> MSVPITRSLQFLRAVHSWLKIARLRSGSYSKLHVTIFRSTPMIRDIIRMGDKRLLRVAPQVTNLGSAELHALVSDMFETMGAAHGVGLAAPQIAVDLQLMVFGFEASERYPEAPAVPLTALANAQIEPLSDEMENGWEGCLSIPGL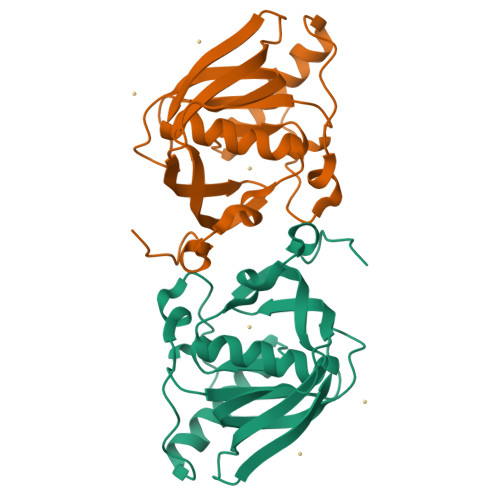RAVIPRYRYIRYRGFAPDGSPIEREAEGFHARVVQHEYDHLVGRLYPSRIENFDTFGFDDVLSYDL>[2x]GPLGSKNHTLYDGQSNGEAKVKKIEFSEFTVKIKNKNNSNNWADLGDLVVRKEEDGIETGLNVGKGDSDTFAGYTATFFSLEESEVNNFIKAMTEGGSFKTSLYYGYKDEQSNANGIQN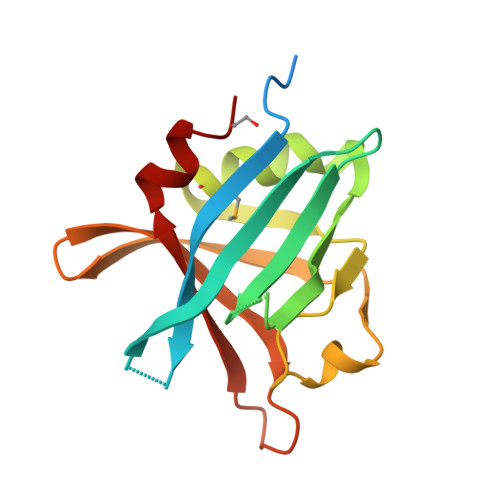KEIITKIEKIDDFEYITFLGDKIKDSGDKVVEYAILLEDLKKNLK>HHHHHHMETKENPWWKKAVVYQIYPKSFKDTTGNGVGDIRGIIEKLDYIKELACDVIWLTPIYQSPQNDNGYDISDYYSIHEEYGTMADFEELLEEAHKRGIKVIMDLVVNHTSTEHRWFKEAASGKENLYRDFYIWKDMKPNGAPPTNWESKFGGSAWEFHAESGQYYLHL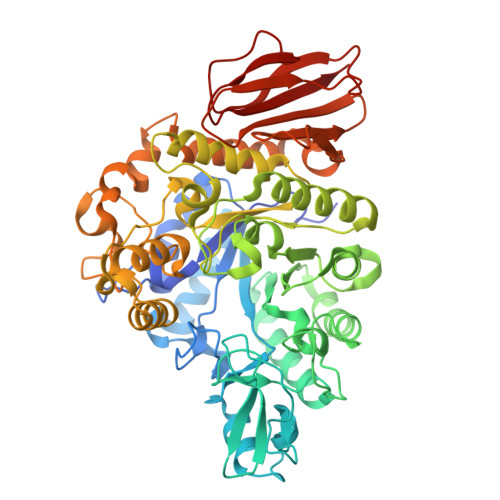YDVTQADLNWENEAVRKKVYEMMHFWFEKGIDGFRLDVINVISKDQRFPDDDEGDGRRFYTDGPRVHEFLNEMNREVFSKYDSMTVGEMSSTTIADCIRYTNPESRELDMVFNFHHLKADYPNGEKWALADFDFLKLKKILSEWQTEMNKGGGWNALFWCNHDQPRIVSRYGDDGKYRKKSAKMLATAIHMLQGTPYIYQGEELGMTNPKFDDISLYRDVESLNMYRILKEAGKPEAEIIEILKAKSRDNSRTPVQWNGEENAGFTAGTPWIPVPDNYKEINAEEALNDPDSIFYHYKKLNELRKEFDIITTGDYQLILEDDQELYAYLRNGADEKLLVINNFYGKETEFQLPDDIDIEGYDAKVLISNDTDLPESFKRFTVKPYQSIVYHLAKPC[4x]> GSASGILLNVKEEVTCPICLELLTEPLSLHCGHSFCQACITANHKKSMLYKEGERSCPVCRIS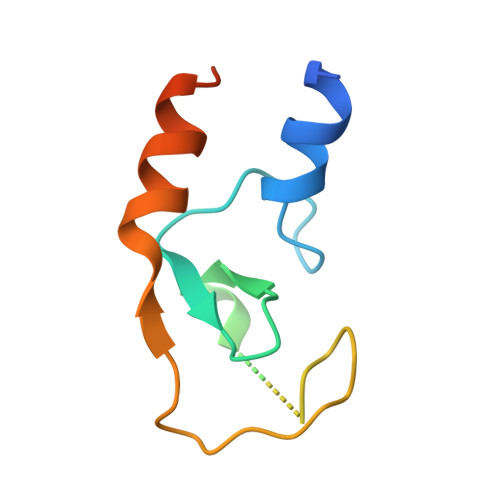YQPENIQPNRHVANIVEKLREVKLSPEEGQ> MSATASTATQPKPLEWLNRLRANPRIPLIVAGSAAVAIVVAMVLWAKTPDYRTLFSNLSDQDGGAIVAQLTQMNIPYRFANGSGAIEVPADKVHELRLRLAQQGLPKGGAVGFELLDQEKFGISQFSEQVNYQRALEGELARTIETLGPVKSARVHLAMPKPSLFVREQKSPSASVTVTLEPGRALDEGQISAVVHLVSSAVAGLPPGNVTLVDQSGHLLTQSNTSGRDLNDAQLKFANDVESRIQRRIEAILSPIVGNGNVHAQVTAQLDFANKEQTEEHYSPNGDASKATLRSRQLNISEQVGAGYPGGVPGALSNQPAPPNEAPIATPPTNQQNAQNTPQTSTSTNSNSAGPRSTQRNETSNYEVDRTIRHTKMNVGDIERLSVAVVVNYKTLADGKPLPLTADQMKQIEDLTREAMGFSDKRGDTLNVVNSPFSAVDNTGGELPFWQQQSFIDQLLAAGRWLLVLVVAWILWRKAVRPQLTRRVEEAKAAQEQAQVRQETEEAVEVRLSKDEQLQQRRANQRLGAEVMSQRIREMSDNDPRVVALVIRQWMSNDHE;> MSNLSGTDKS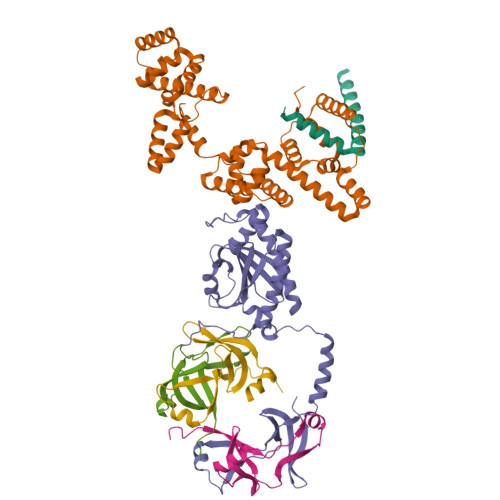VILLMTIGEDRAAEVFKHLSTREVQALSTAMANVRQISNKQLTDVLSEFEQEAEQFAALNINANEYLRSVLVKALGEERASSLLEDILETRDTTSGIETLNFMEPQSAADLIRDEHPQIIATILVHLKRSQAADILALFDERLRHDVMLRIATFGGVQLAELTEVLNGLLDGQNLKRSKMGGVRTAAEIINLMKTQQEEAVITAVREFDGELAQKIIDEMFLFENLVDVDDRSIQRLLQEVDSESLLIALKGAEPPLREKFLRNMSQRAADILRDDLANRGPVRLSQVENEQKAILLIVRRLAETGEMVIGSGEDTYV;> MGDSILSQAEIDALLNGDSDTKDEPTPGIASDSDIRPYDPNTQRRVVRERLQALEIINERFARQFRMGLFNLLRRSPDITVGAIRIQPYHEFARNLPVPTNLNLIHLKPLRGTGLVVFSPSLVFIAVDNLFGGDGRFPTKVEGREFTHTEQRVINRMLKLALEGYSDAWKAINPLEVEYVRSEMQVKFTNITTSPNDIVVNTPFHVEIGNLTGEFNICLPFSMIEPLRELLVNPPLENSRHEDQNWRDNLVRQVQHSELELVANFADIPLRLSQILKLKPGDVLPIEKPDRIIAHVDGVPVLTSQYGTVNGQYALRVEHLINPILNSLNEEQPK;>[3x]MSDMNNPSDENTGALDDLWADALNEQKATTTKSAADAVFQQLGGGDVSGAMQDIDLIMDIPVKLTVELGRTRMTIKELLRLTQGSVVALDGLAGEPLDILINGYLIAQGEVVVVADKYGVRITDIITPSERMRRLSR>MSSLLVKKLVESATTPMRGSEGAAGYDISSVEDVVVPAMGRIAVSTGISIRVPDGTYGRIAPRSGLAYKYGIDVLAGVIDEDYTGEVKVILYNTTERDYIIKKGDRIAQLILEQIVTPGVAVVLDLSDTARGSGGFGSTGI[2x]

dUTPase (EC 3.6.1.23) is a ubiquitous enzyme that catalyzes the hydrolysis of dUTP to diphosphate and dUMP, the substrate for thymidylate synthetase in dTTP biosynthesis. The 141-amino-acid deoxyuridine triphosphatase (dUTPase) from the algal Chlorella virus IL-3A and its Glu81Ser/Thr84Arg-mutant derivative Mu-22 were crystallized using the hanging-drop vapor-diffusion method at 298 K with polyethylene glycol as the precipitant. We previously generated Mu-22 dUTPase by mutating two IL-3A residues to the corresponding residues from PBCV-1 dUTPase. The presence of these two mutations (Glu81Ser and Thr84Arg), creating the derivative Mu-22 dUTPase, led to an increase in the optimal temperature of the enzyme to 328 K. Here, we conduct structural studies of dUTPases from Chlorella viruses in order to elucidate the molecular mechanisms behind the differences in optimal temperature.

Glycyl-seryl-tagged dUTPases yielded cubic P213 IL-3A crystals with unit-cell parameter a = 105.68 Å and hexagonal P63 Mu-22 crystals with unit-cell parameters a = 132.07, c = 53.45 Å, γ = 120°.> ASELLKYLT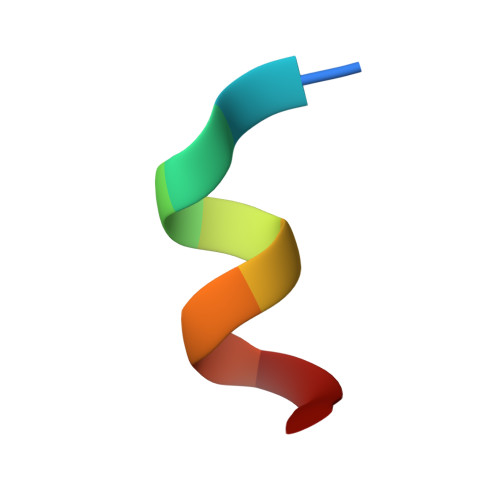T>[2x]MAEIPKEMLRAQTNVILLNVLKQGDNYVYGIIKQVKEASNGEMELNE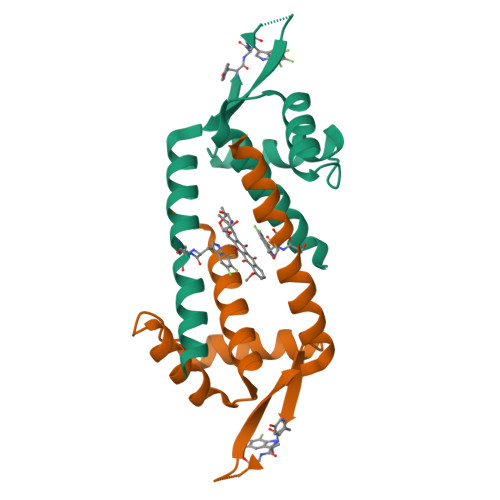ATLYTIFKRLEKDGIISSYXGDESQGGRRKYYRLTEIGHENMRLAFESXSRVDKIIENLEANKKSEAIK> MSAAPVLSITNASVVYPDGISTVTALDSANVEIFPGELVAIVGESGSGKSTLLSIAGFLQEPTSGTVTLHGAEGLDATSTRREHIGFVFQQPNLLGSLTAREQLLITDHLRG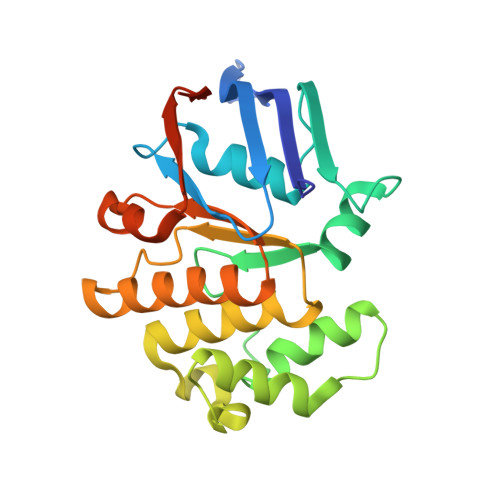IKPRKDRADELLARVGLKGLGGRRVAQLSGGQRQRVNIARALMGNPQLLLADEPTSALDARLSKEIVELLRDVTKEFALATLMVTHDRSQLAYADRFVEMADGKALQTAKLWSHPQFEK We report the 1.8 Å crystal structure of Cass2, an integron-associated protein derived from an environmental V. cholerae. The structure defines a monomeric beta-barrel protein with a fold related to the effector-binding portion of AraC/XylS transcription activators. The closest homologs of Cass2 are multi-drug binding proteins, such as BmrR. Fluorescence assays demonstrate that Cass2 is capable of binding cationic drug compounds with submicromolar affinity.

Structure determination by x-ray crystallography revealed the protein Cass2 to be a monomer organised into a barrel-like form comprising an antiparallel β-sheet of eight strands. The topology of the domain highlights its pseudo two-fold symmetry, which is based on repeating β-β-α-β-β motifs. The central cavity enclosed between the helices of Cass2 is largely hydrophobic in nature, and aromatic side chains predominate. However, a single acidic group (Glu134, originating from strand β7) is buried deep within this cleft, flanking the pseudo two-fold axis of the protein structure. The polarity of this side chain is stabilised by hydrogen bonds to side chains of Tyr56, Tyr136, and Trp111. Between the helical edges of the cavity and directly above the topological switch-point of the sheet (i.e. β3/β7), density is observed corresponding to a polyethylene glycol (PEG) molecule captured during crystallization of Cass2. Hydrophobic side chains from helices α2 (Trp35, Tyr39) and α3 (Pro104, Val107, Ile108, Trp111) and the β7/β8 interstrand loop (Tyr136) are within 4 Å of this ligand. In our structure of Cass2, the site occupied by PEG correlates closely with the location of the cationic drug-binding cavity of BmrR. The loop segment following helix α2 in Cass2 appears to be relatively flexible in our structure, and it is thus feasible that access to the ligand site in the gene cassette domain might occur by a similar helix-opening mechanism, perhaps coupled in this case with expulsion of the interior side chain Tyr39. Despite being a single module, Cass2 retains some of the hydrophobic features of the interface, as well as possessing protruding charged side chains, including Arg149 (as its C-terminal residue).

> MGSSHHHHHHSSGRENLYFQGMNISEINGFEVTGFVVRTTNADEMNPMTAKIGNLWEKFYLNAAPKLTDKSKVYGLYTNYESDFTGAFDVIACSDTLSPQLLSESVKTKVSSGKYVTFSATGEMPQVVIDLWNEVWNYFASEHCPHKRAYTTDFEYYKSANTVEISIAVR>[4x]MA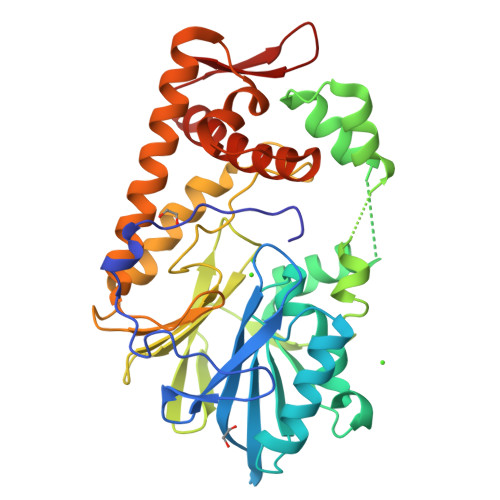HHHHHHMNALEHQLDYPFADGMPAAGTTQEVAPGVYWLRMPLPFALDHINLWLLRDEIDGQKGWTIVDCGIASGEIKANWETVFDTALEGLPVLRVIVTHCHPDHLGLANWLCEGGDKKRWNVRLWITLGEYMLGRVMAAGDGSNAGGEGAARHFARHGLRDEASLDKLRNRKSYYADLVPAVPGQYRRLRDGDALSIGARTWRVVTGFGHSPEHCALHAEADGVLISGDMVLPRISTNVSVFDIEPEGNPLALYLESLGRYETMAADTLVLPSHGKPFRGLHTRIGQLRDHHAARLAEVRAACADKPCSAADIVPIMFRRALDIHQMTFAMGEALAHLHLLWLQGELTRVQGEDGVIRFRA>[2x]MGHHHHHHMNNKPLNTLISATGLWM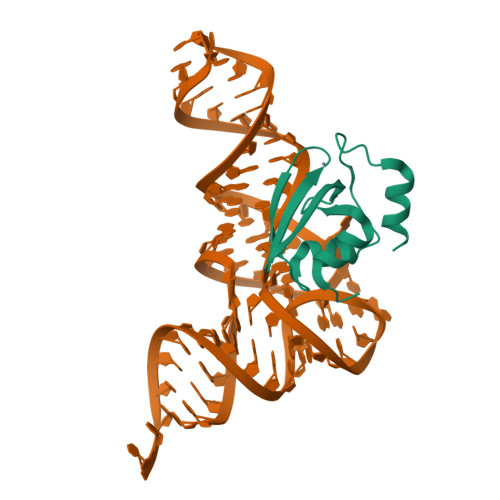SRTGTIHKIKHHEVSRSKIYIEMACGDHLVVNNSRSSRPARALRYHKYRKTCKRCRVSDEDLNKFLTKANEDQTSVKVKVVSAP benzo[c][1,8]naphthyridin-6(5H)-one | C12 H8 N2 O | 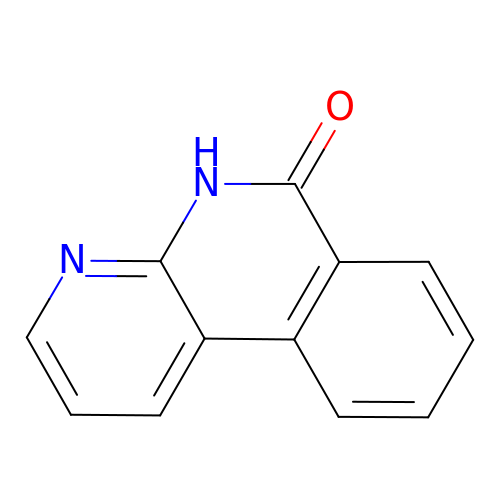YLSBDRGLLZDAKB-UHFFFAOYSA-N>[2x]REKHYYIGITEAVWDYASGSEEKELISVDTEQSNFYLRNGPDRIGRKYKKALYSEYTDGTFTKTIDKPAWLGLLGPVIKAEVGDKVSVHVKNFASRPYTFHAHGVTYTKANEGAIYPDNTTDFQRADDKLFPGQQYLYVLRANEPSPGEGDSNCVTRIYHSHVDAPKDIASGLIGPLILCKKGSLHKEKEENIDQEFVLMFSVVDENLSWYLEDNIKTFCSEPEKVDKDNEDFQESNRMYSINGYTFGSLPGLSMCAEDRVKWYLFGMGNEVDVHSALFHGQALTSKNYHTDIINLFPATLIDVSMVAQNPGVWMLSCQNLNHLKAGLQAFFQVRDCNKPSPDDDIQDRHVRHYYIAAEETIWDYAPSGTDTFTGENLTSLGSDSRVFFEQGATRIGGSYKKLVYREYTDDSFTNRKQRGPDEEHLGILGPVIWAEVGDIIRVTFHNKGQFPLSIQPMGVRFTKENEGTYYGPDGRSSKQASHVAPKETFTYEWTVPKEMGPTYADPVCLSKMYYSGVDLTKDIFTGLIGPMKICKKGSLLADGRQKDVDKEFYLFATVFDENESLLLDDNIRMFTTAPENVDKEDEDFQESNKMHSMNGFMYGNLPGLNMCLGESIVWYLFSAGNEADVHGIYFSGNTYLSKGERRDTANLFPHKSLTLLMTPDTEGSFDVECLTTDHYTGGMKQKYTVNQCKGQFEDVTLYQGERTYYIAAVEVEWDY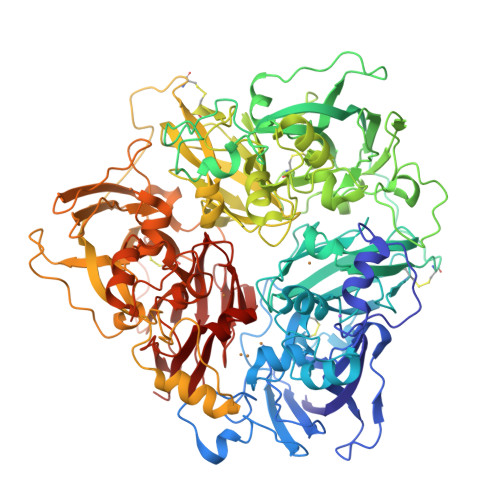SPSRDWEMELHHLQEQNVSNAFLDKEEFFIGSKYKKVVYREFTDSTFREQVKRRAEEEHLGILGPLIHADVGDKVKVVFKNMASRPYSIHAHGVKTKSSTVAPTLPGEVRTYIWQIPERSGAGTEDSPCIPWAYYSTVDRVKDLYSGLIGPLIVCRKSYVKVFNPKKKMEFSLLFLVFDENESWYLDDNINTYSDHPEKVNKDNEEFIESNKMHAINGKMFGNLQGLTMHVGDEVNWYVMAMGNEIDLHTVHFHGHSFQYKHRGIHSSDVFDLFPGTYQTLEMFPQTPGTWLLHCHVTDHIHAGMVTTYTVLPN>[2x]NEGKALMAIKGSFSNLVNMLLDWDD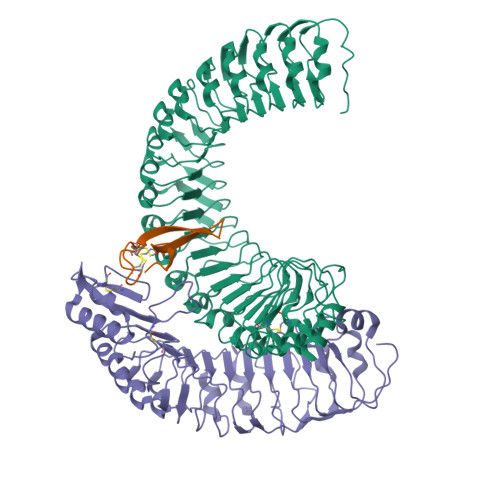VHNSDLCSWRGVFCDNVSYSVVSLNLSSLNLGGEISPAIGDLRNLQSIDLQGNKLAGQIPDEIGNCASLVYLDLSENLLYGDIPFSISKLKQLETLNLKNNQLTGPVPATLTQIPNLKRLDLAGNHLTGEISRLLYWNEVLQYLGLRGNMLTGTLSSDMCQLTGLWYFDVRGNNLTGTIPESIGNCTSFQILDISYNQITGEIPYNIGFLQVATLSLQGNRLTGRIPEVIGLMQALAVLDLSDNELVGPIPPILGNLSFTGKLYLHGNMLTGPIPSELGNMSRLSYLQLNDNKLVGTIPPELGKLEQLFELNLANNRLVGPIPSNISSCAALNQFNVHGNLLSGSIPLAFRNLGSLTYLNLSSNNFKGKIPVELGHIINLDKLDLSGNNFSGSIPLTLGDLEHLLILNLSRNHLSGQLPAEFGNLRSIQMIDVSFNLLSGVIPTELGQLQNLNSLILNNNKLHGKIPDQLTNCFTLVNLNVSFNNLSGIVPPMANFSRFAPASFVGNPYLCGNW;>ARTEPDEQDAVYDIMRATGNDWAAAIPDVCRGRWHGIECMPDQDNVYHVVSLSFGALSDDTAFPTCDPQRSYVSESLTRLKHLKALFFYRCLGRAPQRIPAFLGRLGSSLQTLVLRENGFLGPIPDELGNLTNLKVLDLHKNHLNGSIPLSFNRFSGLRSLDLSGNRLTGSIPGFVLPALSVLDLNQNLLTGPVPPTLTSCGSLIKIDLSRNRVTGPIPESQNRLNQLVLLDLSYNRLSGPFPSSLQGLNSLQALMLKGNNKFSTTIPENAFKGLKNLMILVLSNTNIQGSIPKSLTRLNSLRVLHLEGNNLTGEIPLEFRDVKHLSELRLNDNSLTGPVPFERDTVWRMRRKLRLYNNAGLCVNRDSDAAAAF[2x];>[2x]AGSRLPDCSHACGSCSPCRLVMVSFVCASVEEAETCPMAYKCMCNNKSYPVP> MAKKTSSKGKLPPGPSPLPVLGNLLQMDRKGLLRSFLR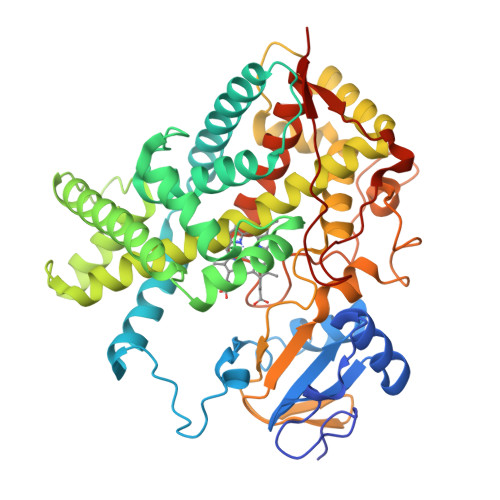LREKYGDVFTVYLGSRPVVVLCGTDAIREALVDQAEAFSGRGKIAVVDPIFQGYGVIFANGERWRALRRFSLATMRDFGMGKRSVEERIQEEARCLVEELRKSKGALLDNTLLFHSITSNIICSIVFGKRFDYKDPVFLRLLDLFFQSFSLISSFSSQVFELFSGFLKHFPGTHRQIYRNLQEINTFIGQSVEKHRATLDPSNPRDFIDVYLLRMEKDKSDPSSEFHHQNLILTVLSLFFAGTETTSTTLRYGFLLMLKYPHVTERVQKEIEQVIGSHRPPALDDRAKMPYTDAVIHEIQRLGDLIPFGVPHTVTKDTQFRGYVIPKNTEVFPVLSSALHDPRYFETPNTFNPGHFLDANGALKRNEGFMPFSLGKRICLGEGIARTELFLFFTTILQNFSIASPVPPEDIDLTPRESGVGNVPPSYQIRFLARHHHH>NRSFSKASGPTQYIFHEEDMNFVDAPTISRVFDEKTMYRNFSSPRGMCLII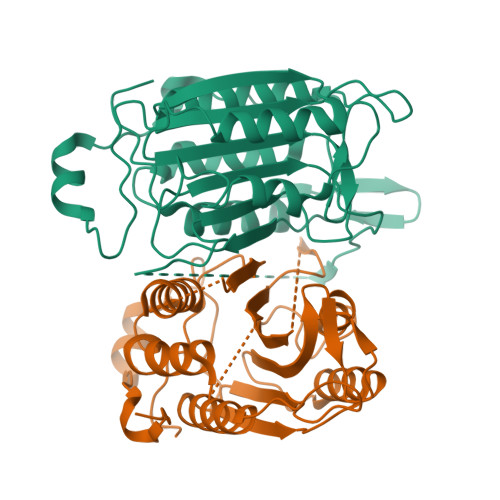NNEHFEQMPTRNGTKADKDNLTNLFRCMGYTVICKDNLTGRGMLLTIRDFAKHESHGDSAILVILSHGEENVIIGVDDIPISTHEIYDLLNAANAPRLANKPKIVFVQASRGERRDNGFPVLDSVDGVPAFLRRGWDNRDGPLFNFLGCVRPQVQQVWRKKPSQADILIAYATTAQYVSWRNSARGSWFIQAVCEVFSTHAKDMDVVELLTEVNKKVACGFQTSQGSNILKQMPEMTSRLLKKFYFWPEARNSAV[2x]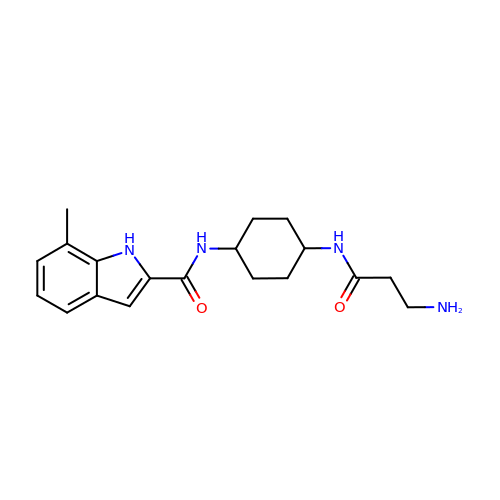N-[(1r,4r)-4-(beta-alanylamino)cyclohexyl]-7-methyl-1H-indole-2-carboxamide | C19 H26 N4 O2 | AEUGFQSECICIPH-SHTZXODSSA-N>MTGDHIKVIYFNGRGRAESIRMTLVAAGVNYEDERISFQDWPKIKPTIPGGRLPAVKITDNHGHVKWMVESLAIARYMAKKHHMMGGTEEEYYNVEKLIGQAEDLEHEYYKTLMKPEEEKQKIIKEILNGKVPVLLDIICESLKASTGKLAVGDKVTLADLVLIAVIDHVTDLDKEFLTGKYPEIHKH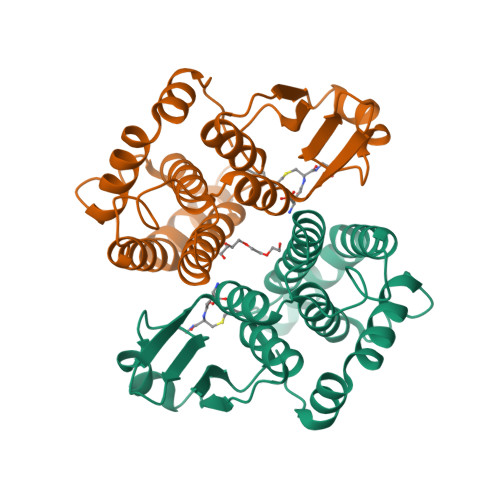RENLLASSPRLAKYLSDRAATPF[2x]>MEEVNLLVLATQYMFWVGFVGMAAGTLYFLVERNSLAPEYRSTATVAALV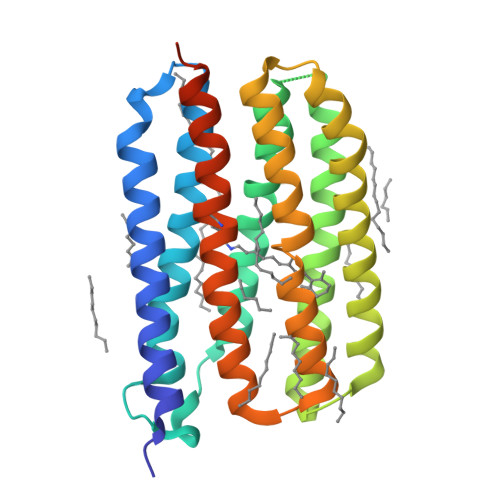TFVAAIHYYFMKDAVGTSGLLSEIDGFPTEIRYIDWLVTTPLLLVKFPLLLGLKGRLGRPLLTKLVIADVIMIVGGYIGESSINIAGGFTQLGLWSYLIGCFAWIYIIYLLFTNVTKAAENKPAPIRDALLKMRLFILIGWAIYPIGYAVTLFAPGVEIQLVRELIYNFADLTNKVGFGLIAFFAVKTMSSLSSSKGKTLTSHHHHHH[2x]> ALEEAPWPPPEGAFVGFVLSRKEPMWADLLALAAARGGRVHRAPEPYKALRDLKEARGLLAKDLSVLALREGLGLPP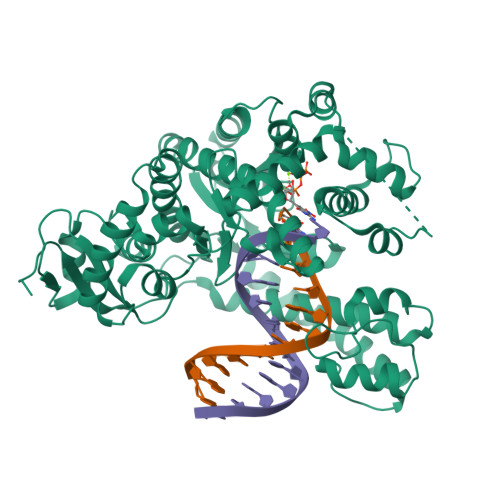GDDPMLLAYLLDPSNTTPEGVARRYGGEWTEEAGERAALSERLFANLWGRLEGEERLLWLYREVERPLSAVLAHVEATGVRLDVAYLRALSLEVAEEIARLEAEVFRLAGHPFNLNSRDQLERVLFDELGLPAIGKTEKTGKRSTSAAVLEALREAHAIVEKILQYRELTKLKSTYIDPLPELIHPRTGRLHTRFNQTATATGRLSSSDPNLQNIPVRTPLGQRIRRAFIAEEGWLLVALDYSQIELRVLAHLSGDENLIRVFQEGRDIHTETASWMFGVPREAVDPLMRRAAKTINFGVLYGMSAHRLSQELAIPYEEAQAFIERYFQSFPKVRAWIEKTLEEGRRRGYVETLFGRRRYVPDLEARVKSVREAAERMAFNMPVQGTAADLMKLAMVKLFPRLEEMGARMLLQVHDELVLEAPKERAEAVARLAKEVMEGVYPLAVPLEVEVGIGEDWLSAKV>LKGQ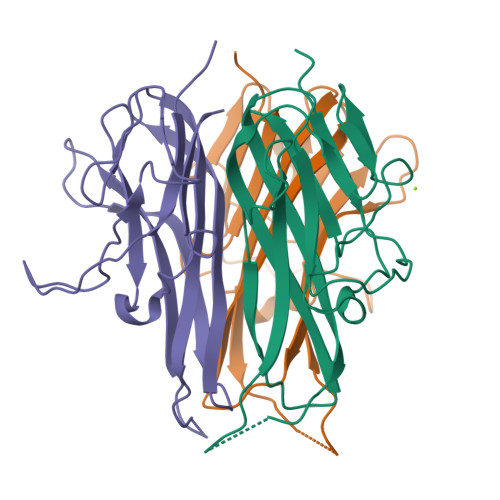EFAPSHQQVYAPLRADGDKPRAHLTVVRQTPTQHFKNQFPALHWEHELGLAFTKNRMNYTNKFLLIPESGDYFIYSQVTFRGMTSECSEIRQAGRPNKPDSITVVITKVTDSYPEPTQLLMGTKSVCEVGSNWFQPIYLGAMFSLQEGDKLMVNVSDISLVDYTKEDKTFFGAFLL[3x]4-FLUORO-2-(4-{[(3S,4R)-4-(1-HYDROXY-1-METHYLETHYL)PYRROLIDIN-3-YL]AMINO}-6,7-DIMETHOXYQUINAZOLIN-2-YL)PHENOL 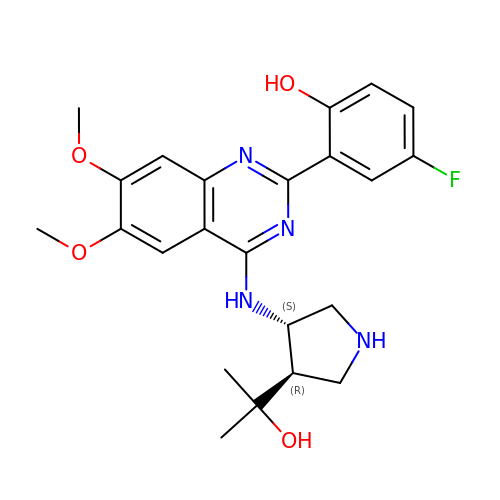| C23 H27 F N4 O4 | HZASIAXCPXTISQ-NVXWUHKLSA-N> TALAEMPKRKFTIDDFDIVRPLGKGKFGNVYLAREKQNKFIMALKVLFKSQLEKEGVEHQLRREIEIQSHLRHPNILRMYNYFHDRKRIYLMLEFAPRGELYKELQKHGRFDEQRSATFMEELADALHYCHERKVIHRDIKPENLLMGYKGELKIADFGWSVHAPSLRRRTMCGTLDYLPPEMIEGKTHDEKVDLWCAGVLCYEFLVGMPPFDSPSHTETHRRIVNVDLK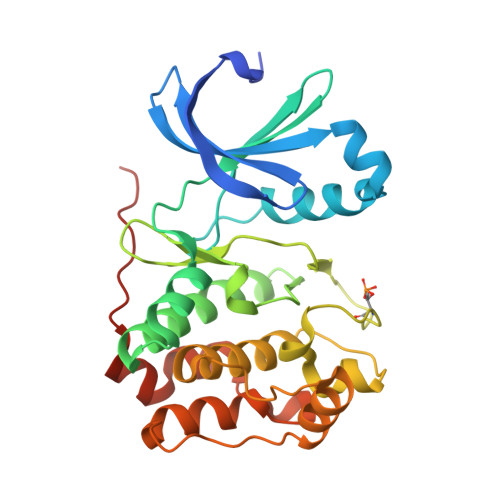FPPFLSDGSKDLISKLLRYHPPQRLPLKGVMEHPWVKANSRRVLPPVYQSTQSK>[2x]MAHHHHHHMAVDAPPAAQGLTNPVDLYPKPPFPHQVQAPPGLASRMQPRPDHGEQSYRGRGRLVGRKTLVT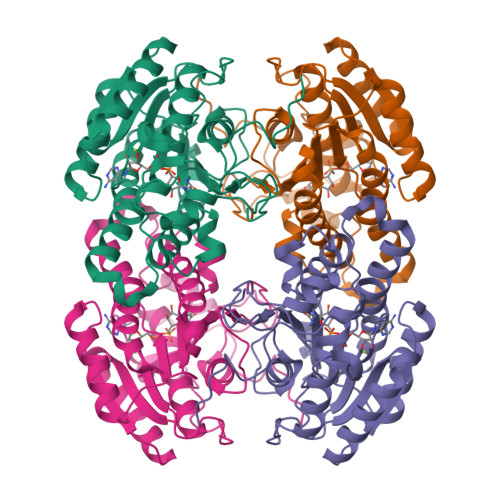GGDSGIGRAAAIAFAREGADVAIGYLPVEESDAREVVALIRAAGRQAVALPGDIRDETFCQRLVARAAEALGGLDILVNNAARQQALDSIGEMTTEHFDATVKTNLYGMFWITKAAIPHLPPGASIINTTSVQAVRASANLLDYATTKAGIIAFTRSLAKQLGPRGIRVNAVAPGPYWTPLQSSGGQPPETVVNYAAGSPYGRPGQPAEIAPLYVALAASETSYANGQVWGADGGLGIF>[4x]PMLKNVVVVGGGTAGWMTASYLTAAFGDRIGVTLVESKRVGSIGVGEATFSTVRHFFEYLGLEEKEWMPACNATYKLAIRFENWREPGHHFYHPFERQRVVDGFPLTDWWLREPRSDRFDKDCFLVGTLCDDLKSPRQLNGELFEGGLGGRSAYRTTLAEQTTQFPYAYHFDATLVANYLRDYAVARGVKHVLDDVQDVALDDRGWISHVVTGESGNLTGDLFIDCTGFRSLLLGKALAEPFQSYQDSLPNDSAVALRVPQDMENRGLRPCTTATAQEAGWIWTIPLFDRIGTGYVYAGDYISPEEAERTLRAFVGPAAEHADANHIKMRIGRSNRHWVNNCVAVGLSSGFVEPLESTGIFFIQH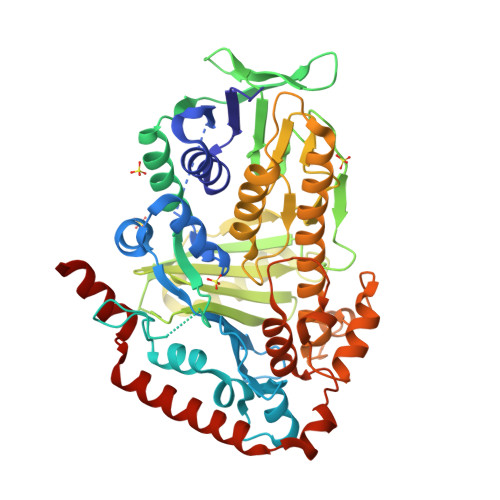AIEQLVKHFPDERWDDGLRTAYNKLVNNVMDGVREFLVVHYYAAKRQDNQYWKDAKTRPLPDGLAERLERWQTRLPDNESVFPHYHGFESYSYVCMLLGLGGLDLKSSPALGLMDAAPARHEFKLVGEQAAELARTLPTQYEYFAQLHRAR>MKKLLALGLLGLVLASCGKKEETTTGPKETTIFAMHLGKALDPNLPVFVKAEKDTNIKLVNVASQNQTDQIQAYNLMLTEGKLPDIVSYELSADLENLGIEGGLIPLEDLINQHAPNLKKFFEENPRYKKDAVAVDGHIYMIPNYYDYFNIKVSQGYFIRQDWLEKLGLKEPRTVDELYTTLKAFREKDPNGNGKKDEVPFFVRANNVRKVLTSLVDLFKASPIWYEENGMVKYGPAQKEFKHAIKELSKWYKEGLIDEEIFTRGLESRDYLLSNNLGGATDDWIASTSSYNRNLADKIPGFNLKLVLPYELNGNAKTRHARTTYLGGWGISKDAKDPVSLIKYFDYWYSVEGRRLWNFGIEGSEYTLVDGKPVFTDKVLKNPDGKTPLAVLREVGAQYRLGAFQDAQYELGWASESAKAGYKYYMDNDVVLDELPILKYTKEKSKEFVSIDTAMRAVVEEKAQQWILGS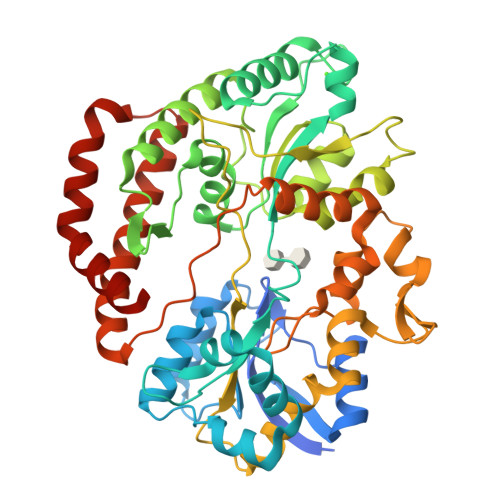GDIDKEWDAYIKRLENLGLSKAEQIQNEAFKNFNK[4x]> LSNLPRVKHTLVPPPFAHAHEQVAASGPVINEFEMRIIEKEVQLDEDAYLQAMTFDGSIPGPLMIVHEGDYVELTLINPPENTMPHNIDFHAATGALGGGGLTLINPGEKVVLRFKATRAGAFVYHCAPGGPMIPWHVVSGMAGCIMVLPRDGLKDHEGKPVRYDTVYYIGESDHYIPKDEDGTYMRFSDPSEGYEDMVAVMDTLIPSHIVFNGAVGALTGEGALKAKVGDNVLFVHSQPNRDSRPALIGGHGDLVWETGKFHNAPERDLETWFIRGGTAGAALYKFLQPGVYAYVNHNLIEAVHKGATAHVLVEGEWDNDLMEQVVAP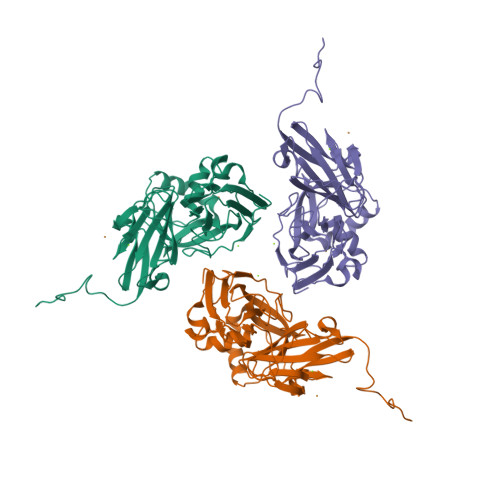VGLTG> LTGPLMLDTAPNAFDDQYEGCVNKMEEKAPLLLQEDFNMNAKLKVAWEEAKKRWNNIKPSRSYPKGFNDFHGTALVAYTGSIAVDFNRAVREFKENPGQFHYKAFHYYLTRALQLLSNGDCHSVYRGTKTRFHYTGAGSVRF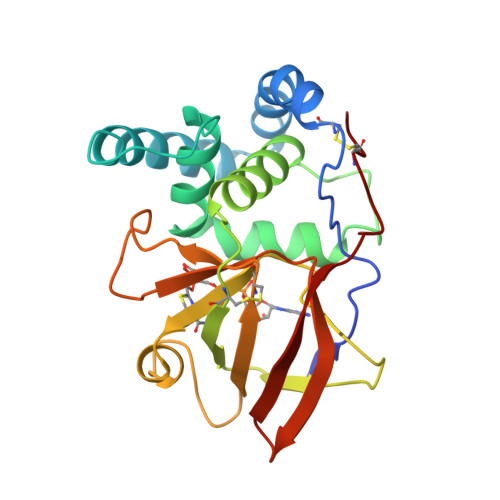GQFTSSSLSKKVAQSQEFFSDHGTLFIIKTCLGVYIKEFSFRPDQEEVLIPGYEVYQKVRTQGYNEIFLDSPKRKKSNYNCLYS> SNAMIRNIVFDLGGVLIHLNREESIRRFKAIGVADIEEMLDPYLQKGLFLDLESGRKSEEEFRTELSRYIGKELTYQQVYDALLGFLEEISAEKFDYIDSLRPDYRLFLLSNTNPYVLDLAMSPRFLPSGRTLDSFFDKVYASCQMGKYKPNEDIFLEMIADSGMKPEETLFIDDG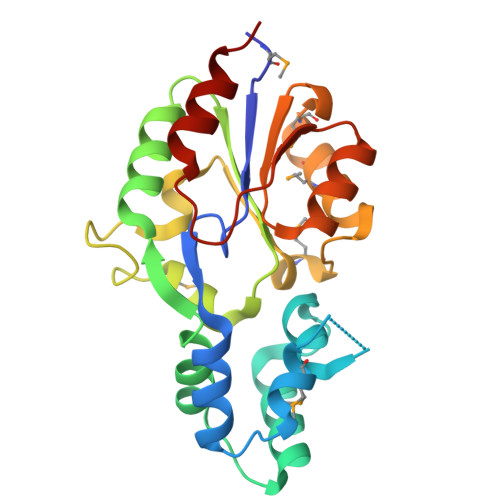PANVATAERLGFHTYCPDNGENWIPAITRLLREQK3-(4-methoxyphenyl)-~{N}-[(3~{R})-1-pyridin-4-ylpyrrolidin-3-yl]-[1,2,3]triazolo[4,5-d]pyrimidin-5-amine | C20 H20 N8 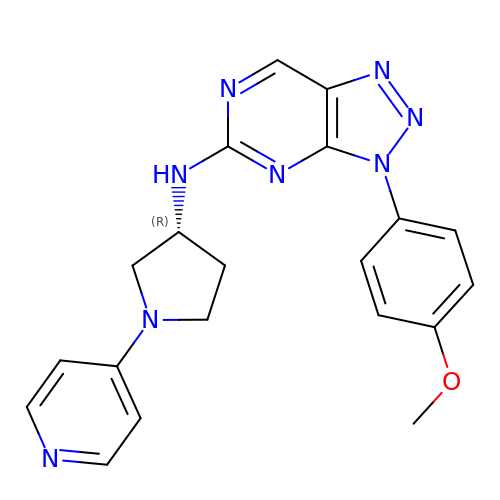O | GDSSVNNRCKMPPZ-CQSZACIVSA-N P. gingivalis is a heme auxotroph, therefore it must acquire this compound to survive and cause efficient infection establishment. Amongst well-characterized heme acquisition systems of P. gingivalis is that encoded by the hmu operon, comprising HmuR, a typical TonB-dependent receptor involved in heme transport across the outer membrane, HmuY, a heme-binding protein, and four proteins with unknown function. The work presented here substantially extends our knowledge of P. gingivalis HmuY by presenting data on further structural characterization of this protein and novel data on a second member of P. gingivalis HmuY-like family, Tfo produced by T. forsythia. The comparative analyses of HmuY homologs suggest that not only the HmuY hemophore-like protein of P. gingivalis, but also T. forsythia Tfo may be engaged in heme acquisition.

Similar to apo-HmuY, apo-Tfo exhibited topology typical of all-β strand structure, with the main distinction apparent in the fold forming the heme-binding pocket, where two long β-strands in HmuY that form one side of the pocket are replaced in Tfo by four shorter β-strands. As compared with apo-HmuY, analysis of the 3D structure of apo-Tfo confirmed differences revealed by spectroscopic analyses, mainly in the fold forming the heme-binding pocket and the lack of two His residues coordinating heme in HmuY. Tfo lacks the two His residues that are required for axial ligation of the heme in HmuY. Instead, Met, Lys, and Tyr residues are potentially available for binding the heme. Based on spectroscopic studies, we assumed that two methionine residues are the best candidates. Although the apo-Tfo structure exhibited a ‘closed’ form, partly caused by malonate binding, MD showed that it could open up to accommodate the heme. Comparison of apo-HmuY with apo-Tfo showed the same kind of opening of this region and it is the ‘same’ loop, containing Met149 (Met169 according to the numbering of amino acid residues in the full length protein) that moves significantly compared with the crystal structure of the closed conformation of apo-Tfo. Importantly, they demonstrated that heme can be bound to Tfo efficiently under reducing conditions, which favors coordination through Met residues. Moreover, reduced conditions influence properties of iron coordination to methionine more significantly than to histidine, thus allowing efficient heme binding also to Tfo and heme sequestration from the albumin-Fe(II)heme complex by Tfo. This effect could be explained by bis-Met heme ligation in Tfo, which results in stabilization of the reduced state as compared with bis-His ligation in HmuY. However, to date we do not have structure of the holo-Tfo, as 1.8 Å data collected from brown holo-Tfo crystals only reveal presence of the apo-form of the protein.

> MDKKDDVKETIKKSKTIDATKYEMWTYVNLETGQTETHRDFSEWHVMKNGKLLETIPAKGSEADIKIKWHIAIHRFDIRTNEGEAIATKETEFSKVTGLPAGDYKKDVEIKDKMLVGFNMADMMKSKFTVAGMAKVNPVLKTWIVENPMGKAPVLSKSVFVVKFKDGSYAKIKFTDATNDKQEKGHVSFNYEFQPK>AQSMNINQEQLLMFQAVMETGSFSAAARKLGKVPSAVSMSIANLEIDLNLTLFERKGREPTPTAEARVLYEKTAQL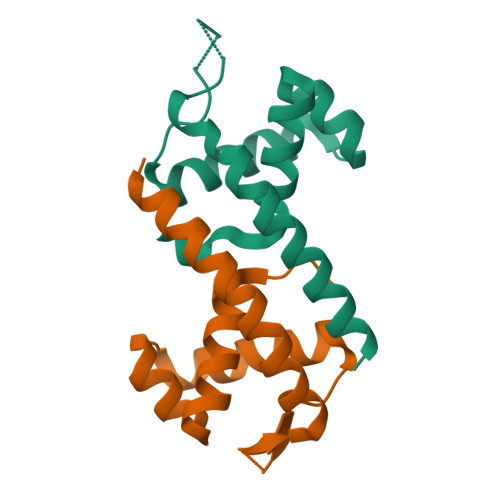LIEMNQWKQHAHAL[3x]>[2x]MASRGVNKVILVGNLGQDPEVRYMPSGGAVA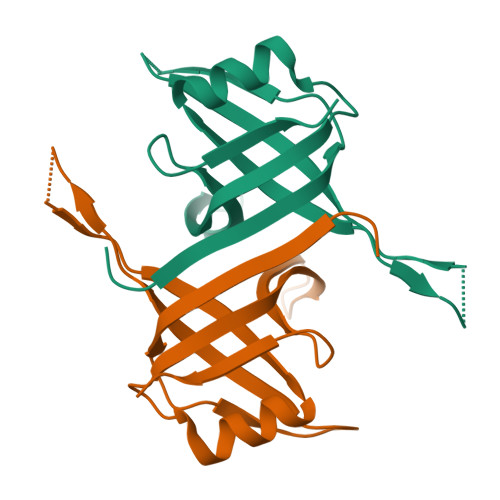NLTLATSESWRDKQTGEMKEQTEWHRVVMFGKLAEVAGEYLRKGSQVYIEGQLRTRKWTDQSGQERYTTEINVPQIGGVMQMLGGHHHHHH> ESKEGSRSSKAKLQISVARSERLLREHGGCSRVSEGAAVALAAAIEYFMGEVL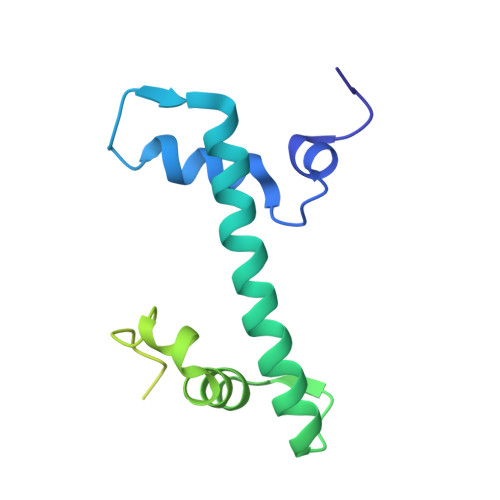ELAGNAARDSKKVRISVKHITLAIQNDAALFAVVGKGVFSGAGVSLISVPIPRKKARKTTEKEASSPKKKAAPKKKKAASKQKKSLSDKELAKLTKKELAKYEKEQGMSPGY>MTMYVIKRSGRKEKLDINKIRIAIKFACEGLNVDPLELEADAQIQFRDGITTKEIQQLLIKTAAEKVSAERPDWTYTAARLLLYDLYKDVAHLRGYSLRDDLGKYKPYNRKNFYSFVKEYVEKGIYGEYLLENYSEEDFNKLANYIKPERDLYFTYTGIKILYDRYLVRDEEGRVIELPQEMYMLIAMTLAVPEKPEERLKWAKKFYDVLSEHKVTVATPTLMNARRPFTQLSSCFVLTVDDDLFDIFDNVKKAGMISKFAGGLGVYLGKIRATGAPIRKFKGASSGVIPVVKLINDTMTYVDQLGMRKGSASITLDIWHKDILDFLEVKTNVGDERKKAHDIHPAVSIPDLFMKRLKNREDWTLIDPYWARQYITRKIYDGKYKEVKPLPGSHYYVGIKEDGTQDILEPKGLEDFYGEEFEKWYLELEENLPSYAKKKVNSFELWKRLLTVAFETGEPYIFFRDEANRKNPNKHTGMVYSSNLCHEIVQTMSPSKHEKPVLDPETGEITYKKEAGDLPVCNLGSVNLGKVHTEEEIKEVLPLLVRMLDNVIEMNFYAIPEAEYTNKRYRAIGIGVSNYHYCLVKNGIKWESEEHLKFADKLFELIAFYALKGSLELAKERGRYKLFDGSNWSKGILFGRSVEEIEENSRQNGNNLPWRELAEEIKKYGIRNAYLLALMPTGSTSLILGATPSIDPIFARFYKEENMSGILPQVPPEVDRFYWHYKTAYTIDHEWTIRAAAVRQKWIDQAQSLNLFVDPQNIDGPRLSRLYELAWELGLKTIYYLRSRSAMDIEECEACSV[2x]

pmcThe enzyme ribonucleotide reductase (RNR) synthesizes the deoxyribonucleotides needed for DNA synthesis from their corresponding ribonucleotide precursors. Class I RNRs are composed of two proteins, a large α-subunit (R1) and a smaller β-subunit (R2) that exist as homodimers, that combine to form an active heterotetramer. Aquifex aeolicus is a hyperthermophilic bacterium with an unusual RNR encoding a 346-residue intein in the DNA sequence encoding its R2 subunit. We present the first structures of the A. aeolicus R1 and R2 (AaR1 and AaR2, respectively) proteins as well as the biophysical and biochemical characterization of active and inactive A. aeolicus RNR.

The structure of AaR1 in complex with ATP was determined to 2.70 Å resolution. The tertiary structure of AaR1 is a homodimer, where each monomer contains an “ATP cone” that houses two ATP molecules. The AaR1 ATP cone has electron density consistent with the presence of two ATP molecules, which is highly unusual, as R1 enzymes generally bind only a single ATP ligand in their ATP cones. The second ATP molecule (ATP2) binds the AaR1 ATP cone in a manner very different from that of ATP1. The adenine base is positioned by a π-stacking interaction between Phe26 and Tyr105, a CH/π interaction with Tyr84, and an interaction between the N7 position and the side chain of Arg99. In the ATP cone, there is also a single magnesium ion, which exhibits octahedral coordination with the phosphate groups of both ATP1 and ATP2. The individual AaR1 monomers interact, forming a dimer interface consisting of four α-helices and their associated loop regions, as well as a novel structural feature in which a β-hairpin (residues 495–515) from one monomer interacts with the equivalent β-hairpin structure from the opposing monomer, forming a four-stranded antiparallel β-sheet across the dimer interface. Interestingly, closer structural analysis of the AaR1 β-hairpin revealed a unique π-stacking interaction between the Tyr511 of each monomer, a residue that is not present in other NrdAh sequences. In the AaR1 structure that lacks nucleotides in both the s-site and the c-site, loop 1 (residues 275–289) and loop 2 (residues 303–310) are disordered in both monomers. The two cysteines (Cys235 and Cys521, AaR1 numbering) that are known to become oxidized upon product formation in E. coli R1 form a disulfide bond in the AaR1 structure.> CPCPGGSSCAIVPKTKEVVCTHCPTGTAGKRCELCDDGYFGDPLGSNGPVRLCRPCQCNDNIDPNAVGNCNRLTGECLKCIYNTAGFYCDRCKEGFFGNPLAPNPADKCKACACNPYGTVQQQSSCNPVTGQCQCLPHVSGRDCGTCDPGYYNLQS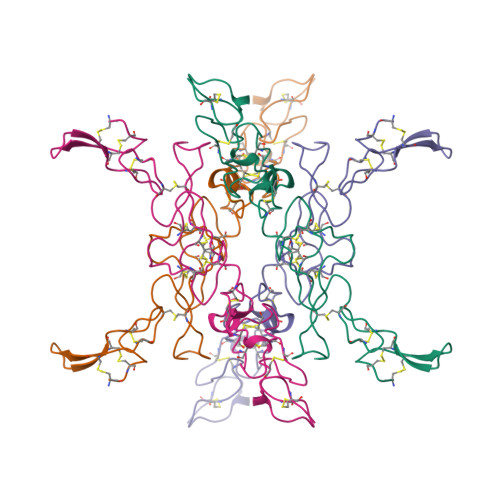GQGCER Here, we identify a PPi-dependent kinase belonging to the ribokinase family, which is distinct from the families of the previously reported PPi-dependent kinases. Accordingly, the phosphate donor specificity of TM0415 was investigated using myo-inositol as the acceptor. This analysis demonstrated that TM0415 utilizes PPi but neither ATP nor ADP to generate myo-inositol monophosphate. Structural comparison and sequence alignment with ATP-dependent or ADP-dependent members of the ribokinase family reveal the importance of five residues: two large hydrophobic residues occluding a part of the ATP-binding pocket and three basic residues specifically involved in PPi recognition. In general, the overall structure of the ribokinase family enzymes is divided into two domains: the phosphate-acceptor-binding domain (the N-terminal half) and the donor-binding domain (the C-terminal half).

We thus also determined the SO42–-complex structure, which possesses only the sulfate ions and myo-inositol in both molecules in an asymmetric unit. The sulfate ion is well superimposed on the distal phosphoryl group of PCP in a protein molecule that crystallographically corresponds to the PCP-bound chain described above. The contribution of R229 to the reaction was confirmed by the fact that an R229A mutant exhibited only 7% of the level of the wild-type activity.

>[2x]MITFIGHVSKDVNVVDGKREIAYGGGVVMGAITSSLLGVKTKVITKCTREDVSKFSFLRDNGVEVVFLKSPRTTSIENRYGSDPDTRESFLISAADPFTESDLAFIEGEAVHINPLWYGEFPEDLIPVLRRKVMFLSADAQGFVRVPENEKLVYRDWEMKEKYLKYLDLFKVDSREAETLTGTNDLRESCRIIRSFGAKIILATHASGVIVFDGNFYEASFRSWSLEGRTGRGDTCTAAFLVGFVFKKMSIEKATKFAAAVTSVKMRHPGPLRREDLEAISGDQYF(R)-1-(4-(4-(HYDROXYMETHYL)-1,3,2-DIOXABOROLAN-2-YL)BENZYL)GUANIDINE 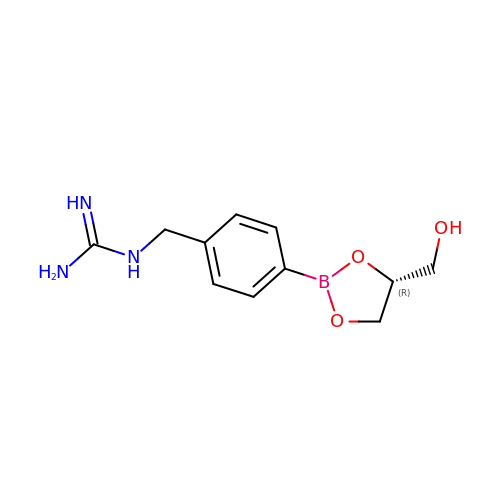| C11 H16 B N3 O3 | IIZOWFNBOXPJES-SNVBAGLBSA-N Neisseria meningitidis is highly adapted to its human host and acquires necessary iron in the host environment using specialized receptor systems that sequester iron from circulating host glycoproteins; notably transferrin (Tf). TbpA functions as a TonB-dependent conduit allowing iron transport through the outer membrane. TbpB extends from the outer membrane surface by virtue of an N-terminal peptide region that is anchored to the outer membrane by fatty acyl chains on the N-terminal cysteine and is involved in the initial capture of iron-loaded Tf. The current study was initiated to explore the sequence and structural diversity of the TbpB and TbpA proteins to gain insights into the covariation and coevolutionary correlations between the TbpA proteins partnered with each TbpB isotype.

The overall approach was to develop structural models for TbpB and TbpA from strain B16B6 to compare to known structures of Tbps from strains with isotype II TbpBs and use this insight to provide a structural context for exploring the sequence diversity of the receptor from of a large collection of N. meningitidis isolates. The overall structural organization was similar, consisting of two orthogonally oriented lobes comprised of N-terminal handle and C-terminal barrel domains. In contrast to the isotype II TbpBs, the loop regions of the handle and barrel domains of the N-terminal lobe were fully resolved in the B16B6 TbpB structure. Similarly, there was only one unresolved loop region in the C-lobe of the B16B6 TbpB compared to four in the type II TbpB structures. Although much of the core secondary structural elements of both isotypes are nearly superimposable, there are subtle differences in loop regions and a tilt of a helix in the N-lobe handle domain (Fig.1C – extended description in Supplementary Section). The primary differences between the TbpB isotypes are present in the unresolved regions of the crystal structure where there is poor electron density in the maps found in the linker region between lobes, and loop regions of the C-lobe (dotted regions – extended description in Supplementary Section). The residues comprising the anchoring peptide that attaches to the outer membrane are not resolved in any of the structures. As revealed by the structural study with the B16B6 TbpB, the most distinct differences between the isotype I and isotype II TbpBs is in the linker region and the C-lobe region where the large loops are reduced or absent in the isotype I TbpB. Isotype I variants also possess longer anchor peptides and shorter linker regions than their isotype II counterparts. The anchor peptide is observed in a locked conformation bound to the C-terminal amino acids of the C-lobe via an antiparallel B strand exchange, while the remaining anchor peptide wraps around the C-lobe domain.

>[3x]SVSENSGAAYGFAVKLPRRNAHFNPKYKEKHKPLGSMDWKKLQRGEPNSFSERDELEKKRGSSELIESKWEDGQSRVVGYTNFTYVRSGYVYLNKNNIDIKNNIVLFGPDGYLYYKGKEPSKELPSEKITYKGTWDYVTDAMEKQRFEGLGSAAGGDKSGALSALEEGVLRNQAEASSGHTDFGMTSEFEVDFSDKTIKGTLYRNNRITQNNSENKQIKTTRYTIQATLHGNRFKGKALAADKGATNGSHPFISDSDSLEGGFYGPKGEELAGKFLSNDNKVAAVFGAKQKDKKDGENAAGPATETVIDAYRITGEEFKKEQIDSFGDVKKLLVDGVELSLLPSEGNKAAFQHEIEQNGVKATVCCSNLDYMSFGKLSKENKDDMFLQGVRTPVSDVAARTEANAKYRGTWYGYIANGTSWSGEASNQEGGNRAEFDVDFSTKKISGTLTAKDRTSPAFTITAMIKDNGFSGVAKTGENGFALDPQNTGNSHYTHIEATVSGGFYGKNAIEMGGSFSFPGNAPEGKQEKASVVFGAKRQQLVQ> MGSSHHHHHHENLYFQGHMENPANANPI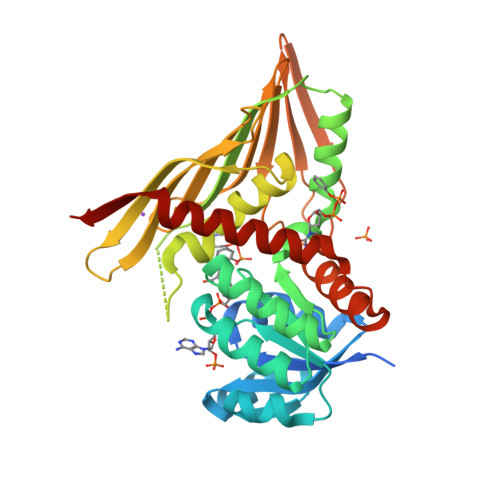RVGVIGCADIAWRRALPALEAEPLTEVTAIASRRWDRAKRFTERFGGEPVEGYPALLERDDVDAVYVPLPAVLHAEWIDRALRAGKHVLAEEPLTTDRPQAERLFAVARERGLLLMENFMFLHHPQHRQVADMLDEGVIGEIRSFAASFTIPPKPQGDIRYQADVGGGALLDIGVYPIRAAGLFLGADLEFVGAVLRHERDRDVVVGGNALLTTRQGVTAQLTFGMEHAYTNNYEFRGSTGRLWMNRVFTPPATYQPVVHIERQDHAEQFVLPAHDQFAKSIRAFAQAVLSGEHPREWSEDSLRQASLVDAVRTGARDIYFP>[2x]MELRKGLEDIAIKETSITYIDGELGRLYYRGYSIFDLASFSNFEEVAYLLWYGKLPTRHELDDFKSRLAEERSISEDISTFVKRTAKFGNPMDIL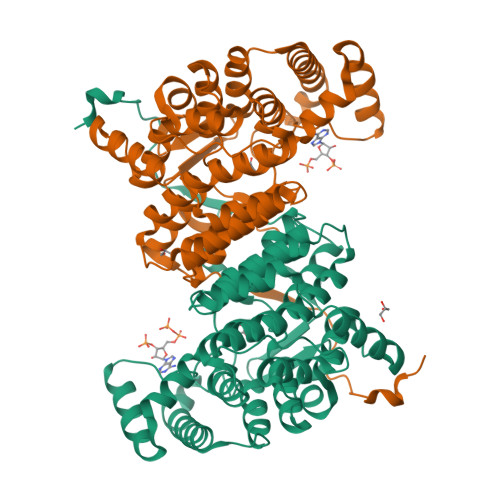RTTVSMMGLEDRSEGDLIGKAIKMTAKIPTIISLIQRTRRNQEFVEPDPSLSHSENFLYMIRGERPSPSDTRVLDVSLMLHMDHEMNASTMACLVVASTLSDIYSSVVAGISALKGPLHGGANSEALKQFMEIETPDNVEKYVMNKLSSGQRLMGFGHRIYKTMDPRAKILKEYANQLSKNEEIKRLFEIANRVEEIGIKILGKRGIYPNVDFYSGLVFYAMGFDPDLFPTIFASARVIGWTAHVDEYLKDNKLIRPKAIYVGDLGKRYVPIEERLEHHHHHH One group of metal ion efflux transporters that regulates metal ion homeostasis and can be found in all domains of life is the Cation Diffusion Facilitator (CDF) protein family. One of the most highly conserved and abundant integral MM proteins is the CDF transporter MamM. MamM was recently proposed to function as a magnetosome-directed iron transporter required for iron biomineralization since its deletion abolished magnetite biomineralization and mutation of residues within the conserved TMD metal-binding site resulted in alterations of magnetite crystal size, morphology and even mineral phase. To summarize our results we present an alternative model for the CDF CTD mode of action, in which we propose that upon metal cation binding, the CTD induces conformational changes towards a tighter and more compact fold which allows the activation of iron transport through the TMD.

Examining this closed state model, three putative binding sites were revealed, in which Asp, Glu and His residues from the two monomers are brought into close proximity and may bind divalent cations. The central binding site is presumed to be the main site as it displays tight packing and contains two symmetry-related His285 and two Asp249 residues. Compared to transcomplementation with the wild-type allele, single point mutations of the histidine residues at the putative central binding site (H285A) or periphery binding sites (H264A) affected neither Cmag values nor the number, size and morphology of the crystals. The D249A, H285A and H264A mutants displayed a minor increase in the number of binding sites compared to the wild-type protein, which may be the result of an increased void volume that allowed the accommodation of additional cations after amino acid substitution to alanine. Fourth, we confirmed metal coordination by the His264 and His285 residues by ssNMR. To confirm that these observed phenotypic differences are due to true transport function alternations, we also examined the expression levels of all MamM mutants, their ability to stabilize MamB expression, performed MD simulations for dimer stability evaluation and determined their CTD structures. (ii) All mutants exhibited an apo-MamM CTD-like behavior along the MD simulations (see Fig. B in file S1 for representative MD simulations), and (iii) an absence of structural differences was observed.

> GSHMEAVQNRIVEAAERVPGVRGVIHLRARYVGQDIWADMIIGVDPENTVEQAHEICEAVQAAVCGKIRRIESLAVSAEAREIGDTTKPSFSDQPLSFDEVMLSKVDN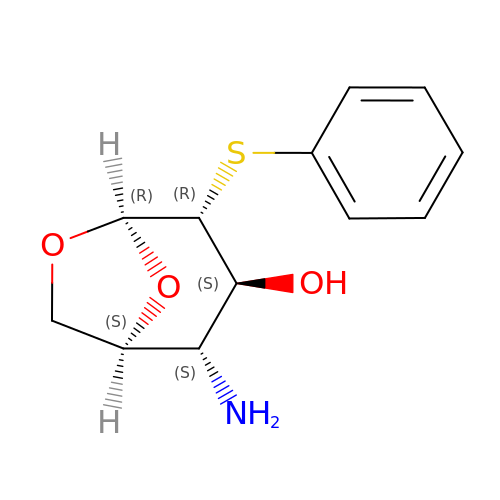(1S,2S,3S,4R,5R)-2-amino-4-(phenylsulfanyl)-6,8-dioxabicyclo[3.2.1]octan-3-ol | C12 H15 N O3 S | OFCUYBHPAYPQJR-RMPHRYRLSA-N>MTKDQNGTWEMESNENFEGYMKALDIDFATRKIAVRLTQTKIIVQDGDNFKTKTNSTFRNYDLDFTVGVEFDEHTKGLDGRNVKTLVTWEGNTLVCVQKGEKENRGWKQWVEGDKLYLELTCGDQVCRQVFKKK[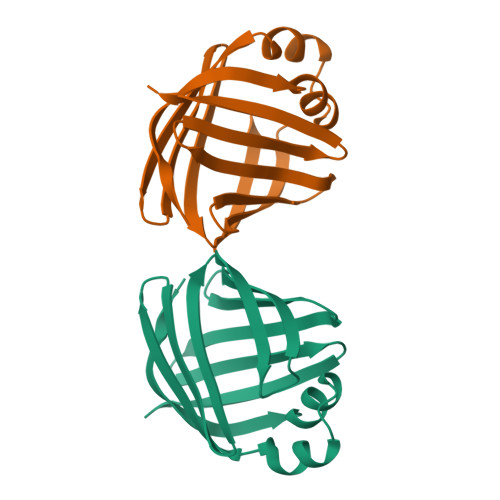2x]> GPPSSLLGAAMPASTSAAALQEALENAGRLIDRQLQEDRMYPDLSELLMVSAPNNPTVSGMSDMDYPLQGPGLLSVPNLPEISSIRRVPLPPELVEQFGHMQCNCMMGVFPPISRAWLTIDSDIFMWNYEDGGDLAYFDGLSETILAVGLVKPKAGIFQPHVRHLLVLATPVDIVILGLSYANLQTGSGVLNDSLSGGMQLLPDPLYSLPTDNTYLLTITSTDNGRIFLAGKDGCLYEVAYQAEAGWFSQRCRKINHSKSSEDDPILQIAIDNSRNILYTRSEKGVIQVYDLGQDGQGMSRVASVSQNAIVSAAGNIARTIDRSVFKPIVQIAVIENSESLDCQLLAVTHAGVRLYFSTCPFRQPLARPNTLTLVHVRLPPGFSASSTVEKPSKVHRALYSKGILLMAASENEDNDILWCVNHDTFPFQKPMMETQMTAGVDGHSWALSAIDELKVDKIITPLNKDHIPITDSPVVVQQHMLPPKKFVLLSAQGSLMFHKLRPVDQLRHLLVSNVGGDGEEIERFFKLHQEDQACATCLILACSTAACDREVSAWATRAFFRYGGEAQMRFPTTLPPPSNVGPILGSPVYSSSPVPSGSPYPNPSFLGTPSHGIQPPAMSTPVCALGNPATQATNMSCVTGPEIVYSGKHNGICIYFSRIMGNIWDASLVVERIFKSGNREITAIESSVPCQLLESVLQELKGLQEFLDRNSQFAGGPLGNPNTTAKVQQRLIGFMRPENG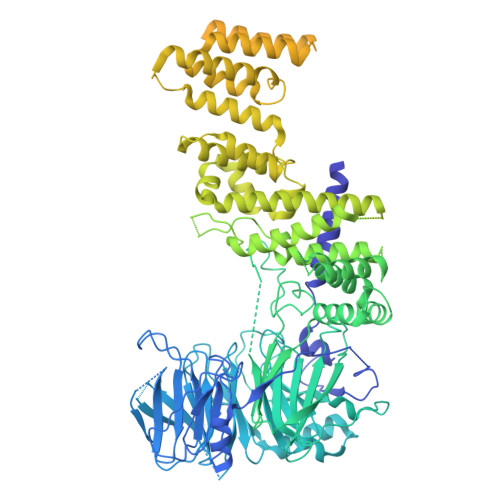NPQQMQQELQRKFHEAQLSEKISLQAIQQLVRKSYQALALWKLLCEHQFTIIVAELQKELQEQLKITTFKDLVIRDKELTGALIASLINCYIRDNAAVDGISLHLQDICPLLYSTDDAICSKANELLQRSRQVQNKTEKERMLRESLKEYQKISNQVDLSNVCAQYRQVRFYEGVVELSLTAAEKKDPQGLGLHFYKHGEPEEDIVGLQAFQERLNSYKCITDTLQELVNQSKAAPQSPSVPKKPGPPVLSSDPNMLSNEEAGHHFEQMLKLSQRSKDELFSIALYNWLIQVDLADKLLQVASPFLEPHLVRMAKVDQNRVRYMDLLWRYYEKNRSFSNAARVLSRLADMHSTEISLQQRLEYIARAILSAKSSTAISSIAADGEFLHELEEKMEVARIQLQIQETLQRQYSHHSSVQDAVSQLDSELMDITKLYGEFADPFKLAECKLAIIHCAGYSDPILVQTLWQDIIEKELSDSVTLSSSDRMHALSLKIVLLGKIYAGTPRFFPLDFIVQFLEQQVCTLNWDVGFVIQTMNEIGVPLPRLLEVYDQLFKSRDPFWNRMKKPLHLLDCIHVLLIRYVENPSQVLNCERRRFTNLCLDAVCGYLVELQSMSSSVAVQAITGNFKSLQAKLERLHSAWSHPQFEK> MRSTCRFFDQTCGPHKSYKYTYMPDPRKLAPIETTTRSEILPLVIRPPTSYVPNHETFLEKVDIHRLKPTSDFKAAFKDWNDLMSCDKRQLRVRGIPRMTRIAIRNAVHAFQNGNPPEYFDTKEEWL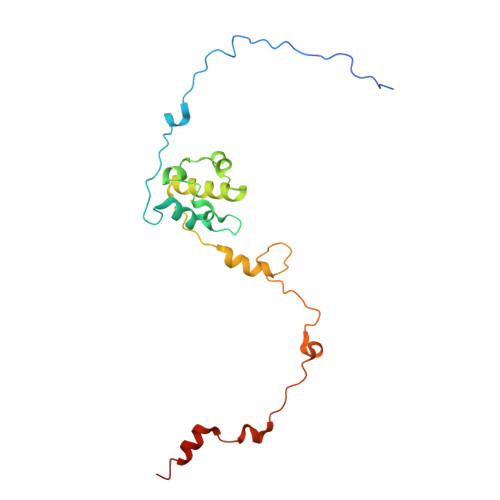YYKQFKTIDFSYRVIPELPEKYRPHQNGIDQAPLPDYREINKMPEWARKEEERLKEKKI> VTEEQVHHIVKQALQRYSEDRIGLADYALESGGASVISTRCSETYETKTALLSLF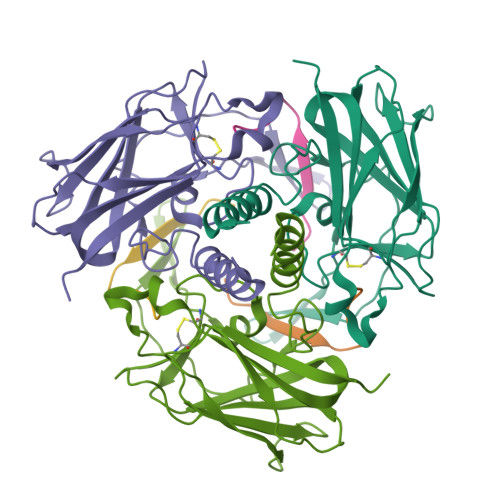GIPLWYHSQSPRVILQPDVHPGNCWAFQGPQGFAVVRLSARIRPTAVTLEHVPKALSPNSTISSAPKDFAIFGFDEDLQQEGTLLGKFTYDQDGEPIQTFHFQAPTMATYQVVELRILTNWGHPEYTCIYRFRVHGEPAH;> FYPMLRYTNGPPPT> MLIQAVGVNLPPSYVCLEGPLGGERPRAQGDEMLMQRLLPAVREALDEAAVKPEEIDLIVGLALSPDHLIENRDIMAPKIGHPLQKVLGANRAHVFDLTDSSLARALYVVDTLASDQGYRNVLVVRGESSQGLEVDSESGFALADGALALLCRPTGKAAFRRGALGGDPAQEWLPLSIPLNTDIRQVGDVKGHLNLPAQPGLPEAVRAGFTRLAGDFPQLNWVREEWFGQGRPDGRCLGPFELASQLRAAQRDRLDELLL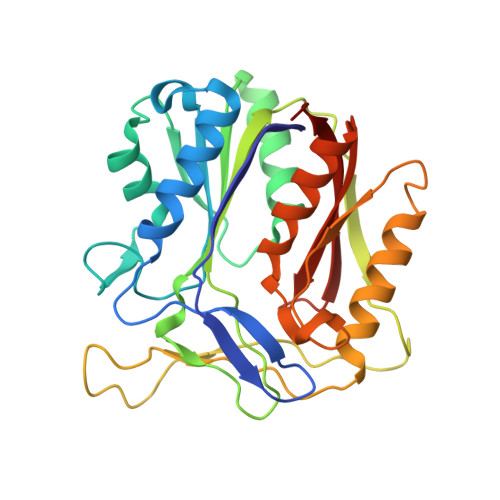ISFDPFGMVVEGVTLELAGEAHA Immunoglobulin E (IgE) is a central regulatory and triggering molecule of allergic immune responses. IgE’s interaction with CD23 modulates both IgE production and functional activities.CD23 is a noncanonical immunoglobulin receptor, unrelated to receptors of other antibody isotypes. Human CD23 is a calcium‐dependent (C‐type) lectin‐like domain that has apparently lost its carbohydrate‐binding capability. The calcium‐binding site classically required for carbohydrate binding in C‐type lectins is absent in human CD23 but is present in the murine molecule.

To determine whether the absence of this calcium‐binding site affects the structure and function of human CD23, CD23 mutant proteins with increasingly “murine‐like” sequences were generated. Restoration of the calcium‐binding site was confirmed by NMR spectroscopy, and structures of mutant human CD23 proteins were determined by X‐ray crystallography, although no electron density for calcium was observed. This study offers insights into the evolutionary differences between murine and human CD23 and some of the functional differences between CD23 in different species.

> SGFVCNTCPEKWINFQRKCYYFGKGTKQWVHARYACDDMEGQLVSIHSPEEQDFLTKHASHTGSWIGLRDLDLEGEFIWVDGSHVDYSNWAPGEPNNGGQGEDCVMMRGSGRWNDAFCDRKLGAWVCDRLATCTPPASEGSAE>MTPAPTPRTDQLHGSRVLVIGGTSGIGFAVCAAALGHGAIVTIVGSNAQKLKDSVARLKSSFPSTDPDDIVAVRCDLSNSDTVEQDIEKALQLAAGNSKINHIVITAADMTAPPPLEDLTVDSVQRPGIIRLVAPLMVAKHLPKYMNKCPQSSLTLTSGAHC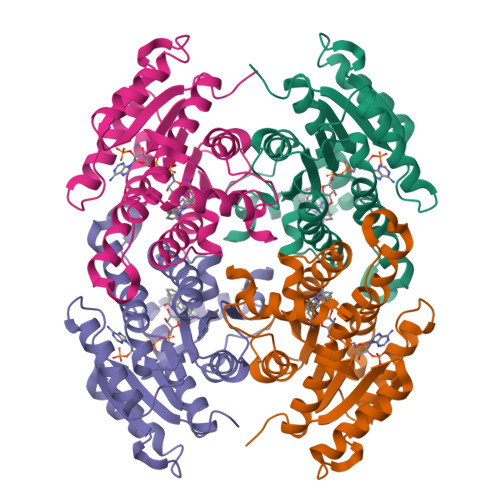LRPDPGWTVISGYCGAVEAMSRGLAIDLKPLRVNVVAPGAVLTEAVKDILGDAYDAAVEMAEAKSTVGQTGSPESVAQAYIYLMKDHYASGSVVSTNGGMLLV[6x]> GGLEKDFLPLYFGWFLTKKSSETLRKAGQVFLEELGNHKAFKKELRHFISGDEPKEKLELVSYFGKRPPGVLHCTTKFCDYGKAAGAEEYAQQEVVKRSYGKAFKLSISALFVTPKTAGAQVVLTDQELQLWPSDLDKPSASEGLPPGSRAHVTLGCAADVQPAQTGLDLLDILQQVKGGSQGEAVGELPRG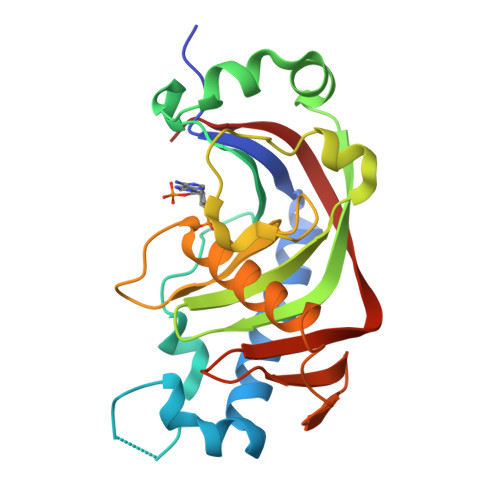KLYSLGKGRWMLSLTKKMEVKAIFTGYYG>[2x]GKHALTGALGNMKKFQSSQKLAQAAMLFMGSKLTTLEETKELTQIFRQLDNNGDGQLDRKELIEGYRKLMQWKGDTV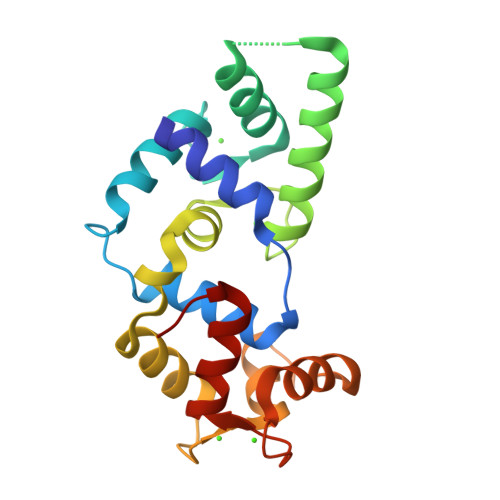SDLDSSQIEAEVDHILQSVDFDRNGYIEYSEFVTVCMDKQLLLSRERLLAAFQQFDSDGSGKITNEELGRLFGVTEVDDETWHQVLQECDKNNDGEVDFEEFVEMMQKICDVKV>[8x]MTPMKTYDLIVIGTGPGGYHAAIRAAQLGLKVLAVEAGEVGGVCLNVGCIPTKALLHAAETLHHLKVAEGFGLKAKPELDLKKLGGWRDQVVKKLTGGVGTLLKGNGVELLRGFARLVGPKEVEVGGERYGAKSLILATGSEPLELKGFPFGEDVWDS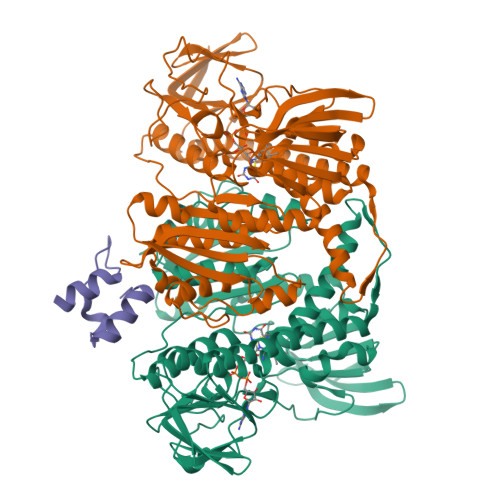TRALKVEEGLPKRLLVIGGGAVGLELGQVYRRLGAEVTLIEYMPEILPQGDPETAALLRRALEKEGIRVRTKTKAVGYEKKKDGLHVRLEPAEGGEGEEVVVDKVLVAVGRKPRTEGLGLEKAGVKVDERGFIRVNARMETSVPGVYAIGDAARPPLLAHKAMREGLIAAENAAGKDSAFDYQVPSVVYTSPEWAGVGLTEEEAKRAGYKVKVGKFPLAASGRALTLGGAEGMVKVVGDEETDLLLGVFIVGPQAGELIAEAALALEMGATLTDLALTVHPHPTLSESLMEAAEAFHKQAIHILNR;>[4x]MLAVPAARKLARELGIPIEEVPGSGPLGRVRVEDVRAYAER>AHMNAGWVIGVDPDTSGALALLKPNQPPQVFDSPHLKVLVGKGVRKRLDAKAIVQLLKSFEAPIGTTVYVEQSTPYPQDGKQGWWSGGFGYGMWIGILVASGFSVIPVPSSAWKSEFQLTKERSNKDYSRQVASQLFPSLSSLLKRKKDHGRAEALLIAAYGKGIKINSDS[2x]

Recently, mutational screening analysis identified the chloroplast-localized HJ resolvase MOC1 that is essential for chloroplast nucleoid segregation in Chlamydomonas reinhardtii and Arabidopsis thaliana. MOC1 exhibits dimerization and an RNaseH fold, belonging to the retroviral integrase superfamily. Moreover, we characterize a base recognition loop (BR loop) that protrudes into the junction and disrupts the C–G base pairs at the crossover. Residue D183 from the BR loop recognizes the cytosine, determining the cytosine-dependent HJ resolution.

After tedious trials, we finally determined two crystal structures of the NtMOC1-HJ complex at an approximately 2.5 Å resolution in the P21212 space group. One of the structures contains the active NtMOC1 and HJ with a noncognate CATG core sequence, and the other is composed of a cleavage-inactive NtMOC1 mutant (D116A/E175A/D253A/E258A) and an HJ with a cognate CCGG core sequence. Here, we use the complex structure of NtMOC1-HJ with a CATG core sequence as a representative to demonstrate the catalytic and binding features. NtMOC1 in the complex also exhibits dimerization, and the HJ is embedded into the cleft of the dimeric NtMOC1. In the HJ-bound complex structure, HJ exhibits an open planar and X-shaped conformation with an overall two-fold symmetry. The center of the junction is opened by NtMOC1 into a parallelogram with cross dimensions of 32 Å between the non-exchanging strands and 9 Å between the exchanging strands. The scissile phosphates are in close proximity to the two active sites of the dimeric enzyme. Four acidic amino acids, namely D116, D118, E175, and E258, coordinate a magnesium ion approach to the cleavable phosphodiester backbone, constituting the catalytic tetrad. More importantly, D183 specifically recognizes the cytosine (C9) via a hydrogen bond. The pairing of D183 (protomer A) to the cytosine (C9, from strand F) led to flipping out of the initially paired guanine (G10, from strand D) from the duplex.>YEQDKTYKITVLHTNDHHGHFWRNEYGEYGLAAQKTLVDGIRKEVAAEGGSVLLLSGGDINTGVPESDLQDAEPDFRGMNLVGYDAMAIGNHEFDNPLTVLRQQEKWAKFPLLSANIYQKSTGERLFKPWALFKRQDLKIAVIGLTTDDTAKIGNPEYFTDIEFRKPADEAKLVIQELQQTEKPDIIIAATHMGHYDNGEHGCNAPGDVEMARALPAGSLAMIVGGHSQDPVCMAAENKKQVDYVPGTPCKPDQQNGIWIVQAHEWGKYVGRADFEFRNGEMKMVNYQLIPVNLKKKVTWEDGKSERVLYTPEIAENQQMISLLSPFQNKGKAQLEVKIGETNGRLEGDRDKVRFVQTNMGRLILAAQMDRTGADFAVMSGGGIRDSIEAGDISYKNVLKVQPFGNVVVYADMTGKEVIDYLTAVAQMKPDSGAYPQFANVSFVAKDGKLNDLKIKGEPVDPAKTYRMATLNFNATGGDGYPRLDNKCGYVNTGFIDAEVLKAYIQKSSPLDV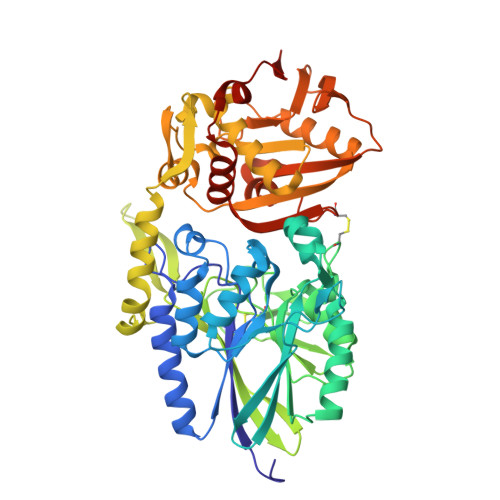SVYEPKGEVSWQEHHHHHH[2x]2-methoxy-4-morpholin-4-yl-aniline | C11 H16 N2 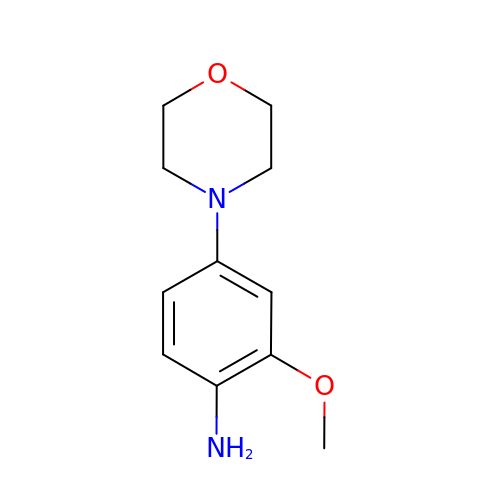O2 | BQTMHUUWYHEPNQ-UHFFFAOYSA-N ethyl 5'-amino[2,3'-bithiophene]-4'-carboxylate | C11 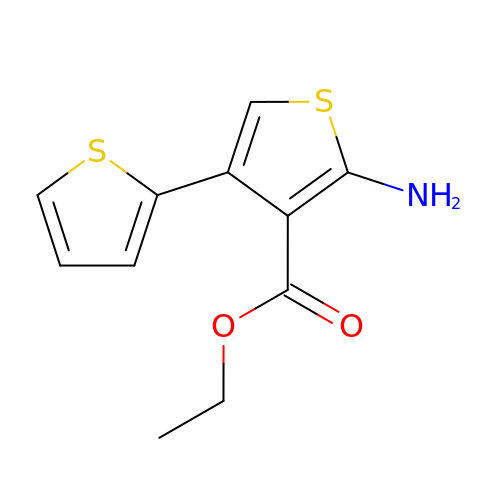H11 N O2 S2 | AKFDBWIUWIWHRK-UHFFFAOYSA-N The transfer of an acetyl group from acetyl-coenzyme A to the free α-amino group on the N-terminus of substrate proteins is catalyzed by N-terminal acetyltransferases (NATs), and is considered to be irreversible, as no Nt-deacetylase has been identified so far. NatC acetylates protein N-termini starting with methionine, followed by a hydrophobic or amphipathic amino acid, with amino acids at positions 3 and 4 also contributing to NatC recognition. NatC forms a heterotrimeric complex, containing the catalytic subunit Naa30, the small auxiliary subunit Naa38 and the large auxiliary subunit Naa35. The large auxiliary subunit Naa35 acts as the central assembly hub of the NatC complex, forming extensive interactions with Naa30 and Naa38.

Structures of the selenomethionine-derivatized (NatC, apo) and native, CoA-bound (NatC•CoA) complex were determined to 2.40 and 2.45 Å resolution, respectively. Both crystallized in space group P212121. The derivatized structures were solved by single-wavelength anomalous diffraction (SAD) and refined to Rwork and Rfree values of 19.5% and 22.3%, respectively. With an RMSD of 0.218 Å, binding of CoA induced only minor structural changes in the catalytic subunit compared to the apo structure. In the peptide-free NatC structures, Leu27 in the α1–α2 loop is positioned in a pocket in between helices α1 and α2. Naa30-Asn147 forms a hydrogen bond with Naa35-Gln106 in the apo and CoA/yArl3-bound NatC structures, but traversed a distance of 8.8 Å in the Gag-bound structure to form an intramolecular hydrogen bond with Naa30-Glu120.

> MEIVYKPLDIRNEEQFASIKKLIDADLSEPYSIYVYRYFLNQWPELTYIAVDNKSGTPNIPIGCIVCKMDPHRNVRLRGYIGMLAVESTYRGHGIAKKLVEIAIDKMQREHCDEIMLETEVENSAALNLYEGMGFIRMKRMFRYYLNEGDAFKLILPLT;> GPMEVDSILGSLSITDDFDQLVDVTSLFDELCSKLKPEAIVKDPRFDLFEGTHSLEVNNSKLDSSLIELTAEEIEFDVNVAYDPPLASVAAIADRLLRCVISWLNDYQTLPTTVLSCRYTESLLSSLVKGTTAGSSWCTGNILYDKVLGSCILGVCYLTKFVQKLLSAGIVFEEEDLNFNNMGFNTFDNLPGQDVVINSLTESLQILEAYSDDSLHLTMLKHILKIIICLVHLEDHLTDYSTKTSHLDELIENANSVNGIFPQLQLSPPKGAFSTYIQKHRSNQFPPRKITKLPTDYSGFITLANDVKTILLVDKAESALETYQFAKFFNKLEQRHVIARILFPLFFIRDDRTVLGKFSYTQFYLLHVKEFSAQTPSEFESSIGNELIQESSNMLLEWYQNCSQNTCRYRQGFNRQLILWDSLQAQFESVNSQVYCSWTYFMKLSSMIEFSLKGFDLDIYKPFEAYSMFWYVYYLSHHLETFLKDSQNDIESNINAIHSMNKKLKKLKAGEKKDQLRLKYRFAMDNEMEQLQATKQFLNYLLKEINITKSLCLIEVFQFAILKSFGLIDNKNSTPSKFSNERLIHNLRFKPFNSIGVPELPEYEVFQQTLKDFVIEEKGAAFDIKLERATNFIETEVRNVVSSIDEIMQGIKGGDNNGVLVTGTRLVQELSLEYYCKLKHTSKALSVNSKVIVNTLKKNIKNKDSHEYKVELVHTTEGWNYFPIQTLRIKQDRYK;> MDILKLSDFIGNTLIVSLTEDRILVGSLVAVDAQMNLLLDHVEERMGSSSRMMGLVSVPRRSVKTIMIDKPVLQELT A cellular pathway has been characterized that performs β-aryl ether (β-ether)3 bond cleavage using three sequential Lig enzymes. The first step in the Lig pathway is a stereospecific oxidation of the benzylic alcohol in the GGE substrate to produce β-(2-methoxyphenoxy)-γ-hydroxypropiovanillone (MPHPV), which is catalyzed by nicotinamide adenine dinucleotide (NAD+)-dependent Cα-dehydrogenases LigD, LigL, LigN, and LigO. The final step consists of a GSH-dependent lyase, LigG, that catalyzes the elimination of the GSH thioether linkage in (βR)-GS-HPV to produce glutathione disulfide (GSSG) and γ-hydroxypropiovanillone (HPV). Our structural and biochemical studies of the enzymes in the bacterial β-aryl ether cleavage pathway reveal the features important for substrate and cofactor binding and catalysis by these Lig enzymes.

The LigD and LigO enzymes catalyze the oxidation of the (αR)-substrates (αR,βR)-GGE and (αR,βS)-GGE, whereas LigL and LigN are specific for the α(S)-configured substrates (αS,βR)-GGE and (αS,βS)-GGE. We have solved the crystal structures of LigD, LigO, and LigL, which by amino acid sequence alignment belong to the short chain dehydrogenase/reductase (SDR) superfamily of enzymes. LigD, LigO, and LigL are classified as classical SDR members that have a core structure of ∼300 residues and share the 11TGXXXGX(G/A)18 sequence motif at the cofactor binding site and the catalytic tetrad N115-S144-Y158-K162 (LigL numbering). The superposition of the LigD, LigO, and LigL structures using Cα atoms shows a root mean square deviation for LigD-LigO of 0.88 Å, for LigD-LigL of 0.70 Å, and for LigO-LigL of 0.93 Å, indicating that the enzymes display similar overall structural features. In these alignments, the most sequence-divergent region is in the predicted substrate binding loop. This proposed substrate binding region is disordered in all of the crystal structures solved in the apo-form (LigD, LigO, and LigL) and in the structures of the LigD·NADH and LigO·NADH complexes. However, in the structures of the binary complex of LigL·NADH and the ternary complex structure of LigL·NADH·(αS,βR)-GGE, this region is well ordered, suggesting that this is a flexible loop that undergoes a major conformational change upon cosubstrate binding to the enzyme.

>[2x]MDIAGTTAFITGGASGIGFGIAQRLLANGARLVLADIRQDHLDEARQFFEERQQGRNVHTIRLDVSDRAQMAEAARECEAVMGGPDILINNAGIDPSGPFKDATYQDWDYGLAINLMGPINGIMAFTPGMRARGRGGHIVNTASLAGLTPMPSFMAIYATAKAAVITLTETIRDSMAEDNIGVTVLMPGPIKSRIHESGQNRPERFRAGSGLAETEQQLAKRVVADNWMEPTEVGDMIVDAIVHNKLYVSTHGNWRETCEARFQALLDSMPEARPFDFGASLAVPKEEA(2~{S})-2-(1-chloranylcyclopropyl)-1-(2-chlorophenyl)-3-(1,2,4-triazol-1-yl)propan-2-ol | 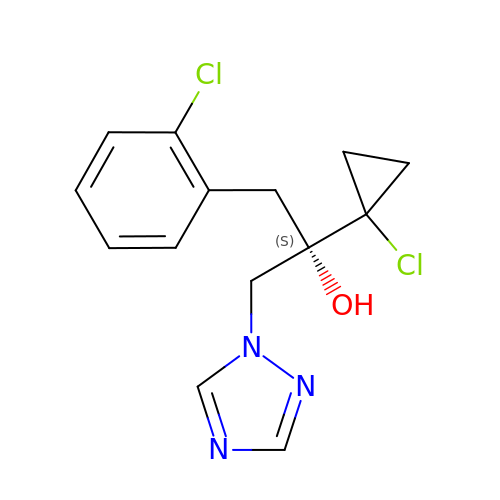C14 H15 Cl2 N3 O | HHUQPWODPBDTLI-AWEZNQCLSA-N>[2x]GPLGSMAQSTVLPMHCLYGIFLEGNLKIQKNDQEGLKKFKDNIKKFTLELDEIDKISPQSRIGGAICFSSDIWDTVTKKISKPKELKSVNTLSSYMPGTSQRDILIHIISDRMDTCFKLAQDTMRNFGEDQLDIKQEIHGFRRVEERDLTDFIDGTENPDGDELRTQYGLVAAGQPNEFGSYVFTQRYVHNLKKWYPEPLSVQQDTVGRTKKDSIEIPRDKRPITSHVSRTDLSENGKDLKIVRQSLPYGQITGEKGLMFIAYACSLHNIEKQLQSMFGQLDGKHDLLLKYTTPVTGSFYFAPSKKELLEL

A novel cytoplasmic dye-decolorizing peroxidase from Dictyostelium discoideum was investigated that oxidizes anthraquinone dyes, lignin model compounds, and general peroxidase substrates such as ABTS efficiently. Dictyostelium DyPA is a dimer, with each monomer exhibiting a two-domain, α/β ferredoxin-like fold. In solution, Dictyostelium DyPA exists as a stable dimer with the side chain of Asp146 contributing to the stabilization of the dimer interface by extending the hydrogen bond network connecting two monomers. The active site of Dictyostelium DyPA has a hexa-coordinated heme iron with a histidine residue at the proximal axial position and either an activated oxygen or CN− molecule at the distal axial position.

The structure of Dictyostelium DyPA in complex with an activated form of oxygen was determined to 1.7 Å resolution. In the asymmetric unit, two molecules of Dictyostelium DyPA were found. The Fe (III) is hexa-coordinated and is in the plane of the porphyrin ring. The heme group has His222 on its proximal side, and the distal side is occupied by Asp149, Arg239, Ser241, Leu253, and Phe255. The sixth coordination position at the distal face of the heme iron is occupied by an activated oxygen molecule with elongated bond distances between the oxygen atoms of 1.7 and 2.4 Å in the two monomers. The observed distances between the coordinated oxygen atom and the heme iron in the two monomers are 2.3 and 2.6 Å. The other oxygen atom is coordinated by a hydrogen-bond network that involves Asp149, Ser241, an ethylene glycol, and water molecules. Electron density analysis revealed excess electron density on the Nδ atom of His222 imidazole, which exceeds the maximum level of electron density on the carboxyl group of Asp281 by ~1σ. This observation suggests that the imidazole ring of His222 is negatively charged in the crystal structure of the Dictyostelium DyPA:O2 complex, while the carboxyl group of Asp281 is protonated. The negative charge on His222 explains the elongated bond length in the activated O2 molecule by the decreasing effect of an additional electron on the energy difference between the highest occupied (HOMO) and lowest unoccupied (LUMO) molecular orbitals of the complex. Arg239 forms hydrogen bonds with the distally positioned heme propionate, Asp149, and the O2 molecule.> MQDVRVQVLPEVRGQLGGTVELPCHLLPPVPGLYISLVTWQRPDAPANHQNVAAFHPKMGPSFPSPKPGSERLSFVSAKQSTGQ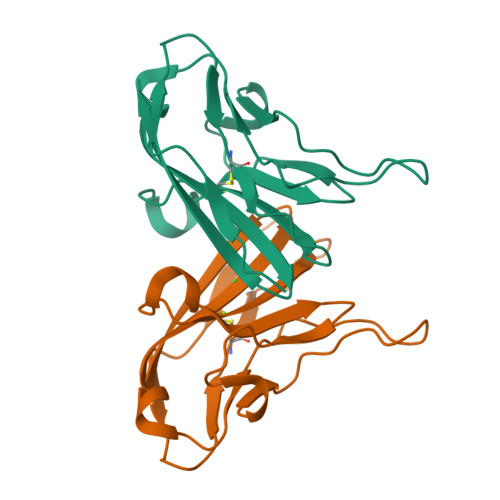DTEAELQDATLALHGLTVEDEGNYTCEFATFPKGSVRGMTWLRV>SNAMSRRLWLRNTLVATALLSVFSVPVSAATHTLQLAIGDEPTEGFDPMLGWSHGSYLLLHSPLLKQNEDFSWDSLLLSQYQPSDDGKTWLLTLKPDLKFSDGSPLTAKDVAFTYNNAAASGGKVDMGNFLSAEVIDPLNVRIHLKAPQSTFVNVLGSLGIVSADKYNAKTYAQKPIGAGPYRLVSFQPGQQMIVEANPYYAGNKNDFDKLIFVFLDEDSAFAAAQSGQLGVVRIPPSMAVGSVNNMKLWVRPSVENRGIVFPTTPAGKKDAHGYPIGNDVTADVAIRRAINYAINRQLLADQIMEGHAIPAYTGVQGLPWNNPDSAIKDGDIDK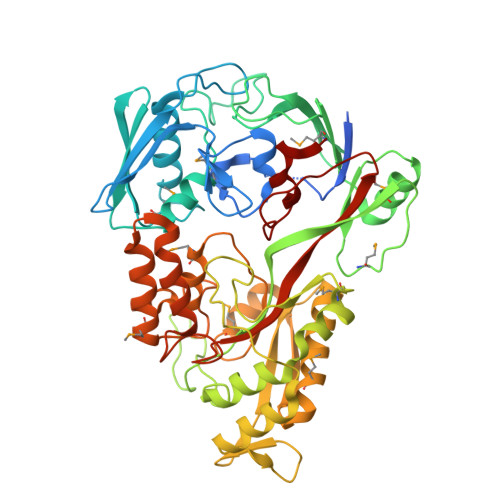AKQILEQAGWQLNSQGTREKNGLPAKITLWYTSGDTTRRDLAQALRSMLKPIGIDVDLKSGSWETVERNMHANPTLFGWGSLDPMELYHHYSSNAAGVEYYNPGYYKNPMVDKHLQQALDAPTWQQAVPFWQQVDWDGTTGAGIRGDAAWAWLLNIQHTYLANNCVDLGKGTPEIHGSWSLLNSIDSWKWTCQ[2x]5-(dimethylamino)-~{N}-[6-[(2~{S},3~{R},4~{S},5~{R})-3-(hydroxymethyl)-4,5-bis(oxidanyl)piperidin-2-yl]hexyl]naphthalene-1-sulfonamide 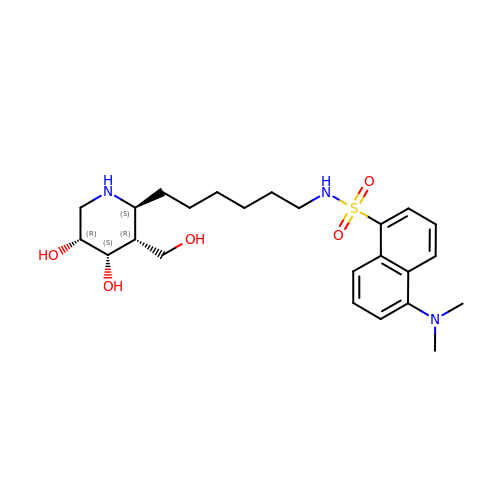| C24 H37 N3 O5 S | YUUSOYGEJQMOTK-QRVLJTFESA-N> MSNLNLFATILTYPAPASNYRGESEENRSVIQKILKDGQKYAIISPESMRNALREMLIELGQPNNRTRLHSEDQLAVEFKEYPNPDKFADDFLFGYMVAQTNDAKEMKKLNRPAKRDSIFRCNMAVAVNPYKYDTVFYQSPLNAGD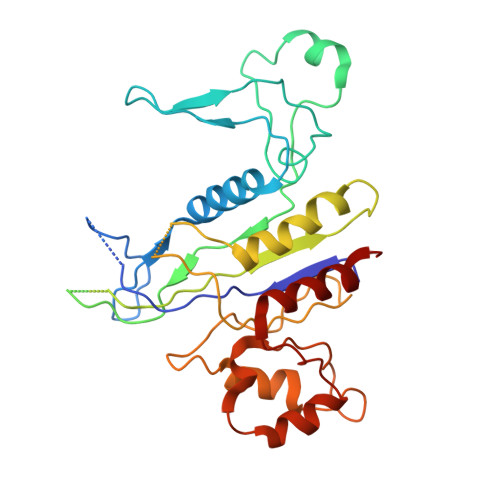SAWKNSTSSALLHREVTHTAFQYPFALAGKDCAAKPEWVKALLQAIAELNGVAGGHARAYYEFAPRSVVARLTPKLVAGYQTYGFDAEGNWLELSRLTATDSDNLDLPANEFWLGGELVRKMDQEQKAQLEAMGAHLYANPEKLFADLADSFLGV> MLVAYDSMTGNVKRFIHKLNMPAVQIDEDLVIDEDFILITYTTGFGNVPERVLDFLERNNEKLKGVSASGNRNWGDMFGASADKISTKYEVPIVSKFELSGTNNDV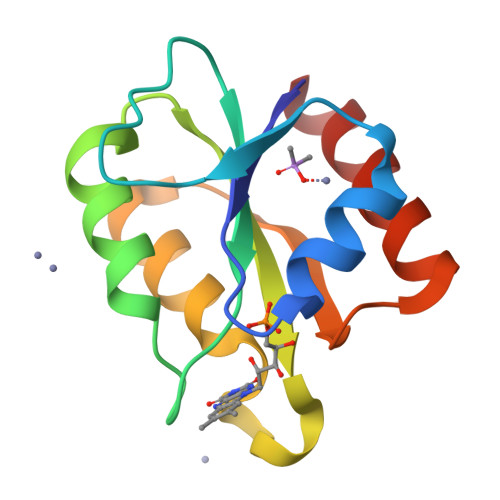EYFKERVREIATH2,5-dimethylpyrazine 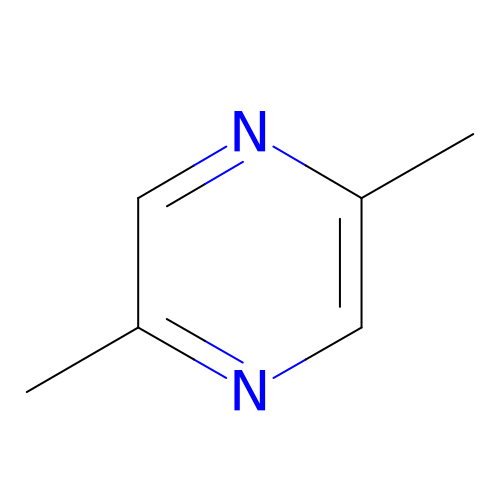| C6 H8 N2 | LCZUOKDVTBMCMX-UHFFFAOYSA-N>MSRNNDINAEVVSVSPNKLKISVDDLEEFKIAEEKLGVGSYLRVSDNQDVALLAIIDNFSIEVKESQKQKYMIEASPIGLVKNGKFYRGGDSLALPPKKVEPAKLDEIISIYSDSIDINDRFTFSSLSLNTKVSVPVNGNRFFNKHIAIVGSTGSGKSHTVAKILQKAVDEKQEGYKGLNNSHIIIFDIHSEYENAFPNSNVLNVDTLTLPYWLLNGDELEELFLDTEANDHNQRNVFRQAITLNKKIHFQGDPATKEIISFHSPYYFDINEVINYINNRNNERKNKDNEHIWSDEEGNFKFDNENAHRLFKENVTPDGSSAGALNGKLLNFVDRLQSKIFDKRLDFILGEGSKSVTFKETLETLISYGKDKSNITILDVSGVPFEVLSICVSLISRLIFEFGYHSKKIKRKSNENQDIPILIVYEEAHKYAPKSDLSKYRTSKEAIERIAKEGRKYGVTLLLASQRPSEISETIFSQCNTFISMRLTNPDDQNYVKRLLPDTVGDITNLLPSLKEGEALIMGDSISIPSIVKIEKCTIPPSSIDIKYLDEWRKEWVDSEFDKIIEQWSKS[6x]

Here, we biochemically and structurally characterize a two-component defense system DUF4297–HerA, demonstrating that DUF4297–HerA confers resistance against phage infection by cooperatively cleaving dsDNA and hydrolyzing ATP. DUF4297 encodes a protein containing an N-terminal DUF4297 domain (a putative PD-(D/E)xK-family nuclease) with predicted yet-to-be biochemically characterized nuclease activity and a C-terminal domain (CTD) with unknown function. HerA, widely distributed in archaea and bacteria, encodes a DNA motor protein, which can hydrolyze ATP and translocate along DNA. The enzymatic activities and anti-phage defense function of the DUF4297–HerA system are activated through supramolecular assembly.

We first determined the cryo-EM structure of HerA alone at an overall resolution of 3.14 Å. The single HerA molecule adopts an elongated structure. It can be divided into three domains from top to bottom: an N-terminal β-barrel domain, also named HAS, which is a characteristic β-barrel fold seen at the bovine F1-ATP synthase and HerA,23,24 the central RecA-like catalytic core (RecA-like), and a flanking four-helix bundle (Helix bundle). Unexpectedly, HerA assembles into a split spiral hexamer with a cleft between the topmost and bottommost subunits. This is in remarkable contrast to previously determined structures of HerA homologs, which form a planar symmetric hexamer. The C-terminal hook docks into the surface grooves of the neighboring subunit to strengthen the HerA oligomerization; however, this interaction is disrupted between the topmost and bottommost subunits, destabilizing the hexamer formation. Interestingly, HerA alone shows extremely low ATPase activity. Structural comparison immediately explains why the ATPase activity of HerA alone is inhibited. While the pocket created by Walk A and Walk B motifs can accommodate the ATP molecule, relocation of the R finger is needed to hydrolyze ATP because it is too far away (20 Å) from the Walker A motif with which they form the ATPase active site. However, the required conformational change would cause a steric clash at the insertion and four-helix bundle domains, hindering the required movement of the R finger.> MRGSHHHHHHGLVPRGSMIRTMLQGKLHRVKVTHADLHY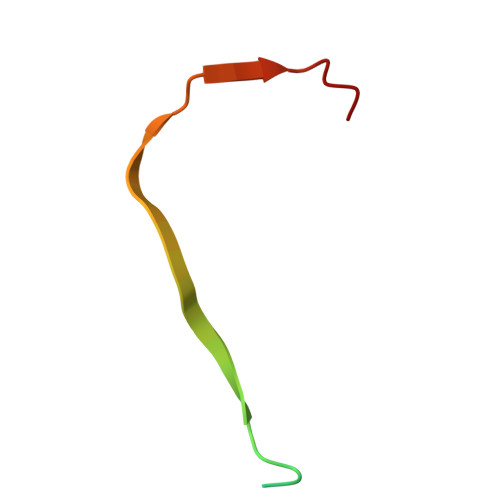EG> MIRLSLFISLLLTSVTVLADVQINIRGHVYIPPCTINNGQNIVVDFGNINPEHVDNSRGEVTKTISISCPYKSGSLWIKVTGNTMGGG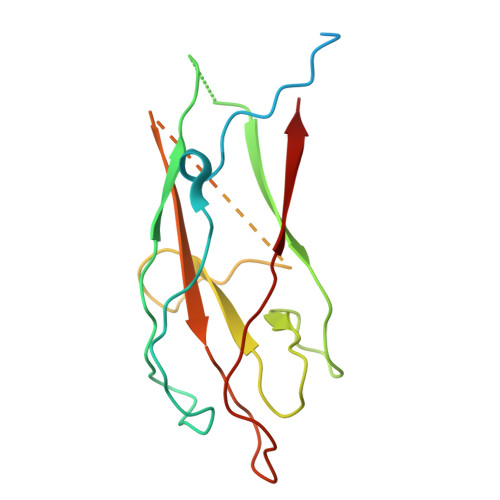QNNVLATNITHFGIALYQGKGMSTPLTLGNGSGNGYRVTAGLDTARSTFTFTSVPFRNGSGILNGGDFRTTASMSMIYN>MRSYEQMETDGERQNATEIRASVGKMIDGIGRFYIQMCTELKLSDYDGRLIQNSLTIERMVLSAFDERRNKYLEEHPSAGKDPKKTGGPIYRRVDGKWRRELILYDKEEIRRIWRQANNGDDATAGLTHMMIWHSNLNDATYQRTRALVRTGMDPRMCSLMQGSTLPRRSGAAGAAVKGVGTMVMELIRMIKRGINDRNFWRGENGRRTRIAYERMCNILKGKFQTAAQRTMVDQVRESRNPGNAEFEDLIFLARSALILRGSVAHKSCLPACVYGSAVASGHDFEREGYSLVGIDPFRLLQNSQVVSLIRPNENPAHKSQLVWMACHSAAFEDLRVSSFIRGTKV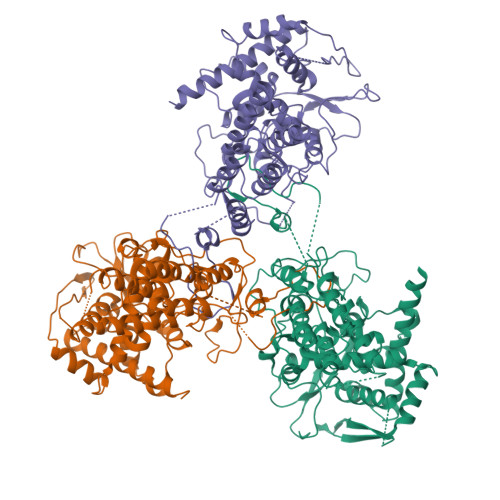VPRGKLSTRGVQIASNENMETMESSTLELRSRYWAIRTRSGGNTNQQRASSGQISIQPTFSVQRNLPFDRPTIMAAFTGNTEGRTSDMRTEIIRLMESARPEDVSFQGRGVFELSDEKATSPIVPSFDMSNEGSYFFGDNAEEYDNLEHHHHHH[3x]>[2x]LYPIAVLIDELRNEDVQLRLNSIKKLSTIALALGVERTRSELLPFLTDTIYDEDEVLLALAEQLGTFTTLVGGPEYVHCLLPPLESLATVEETVVRDKAVESLRAISHEHSPSDLEAHFVPLVKRLAGGDWFTSRTSACGL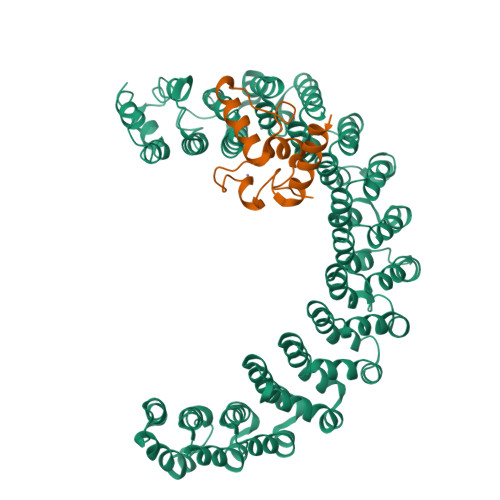FSVCYPRVSSAVKAELRQYFRNLCSDDTPMVRRAAASKLGEFAKVLELDNVKSEIIPMFSNLASDEQDSVRLLAVEACVNIAQLLPQEDLEALVMPTLRQAAEDKSWRVRYMVADKFTELQKAVGPEITKTDLVPAFQNLMKDCEAEVRAAASHKVKEFCENLSADCRENVIMSQILPCIKELVSDANQHVKSALASVIMGLSPILGKDNTIEHLLPLFLAQLKDECPEVRLNIISNLDCVNEVIGIRQLSQSLLPAIVELAEDAKWRVRLAIIEYMPLLAGQLGVEFFDEKLNSLCMAWLVDHVYAIREAATSNLKKLVEKFGKEWAHATIIPKVLAMSGDPNYLHRMTTLFCINVLSEVCGQDITTKHMLPTVLRMAGDPVANVRFNVAKSLQKIGPILDNSTLQSEVKPILEKLTQDQDVDVKYFAQEALTVLSLA;>SLNPGVDAMYCKQWPECAKKMSANCICLLCLLRMKHENRKLYRKDPLVWVDCYCFDCFRMWFGLDLCEGTLLLWCDIIGQTTYRDLKL[2x]>[4x]MGSSHHHHHHSSGGNENLYFQGHMARASGSERHLLLIYTGGTLGMQSKGGVLVPGPGLVTLLRTL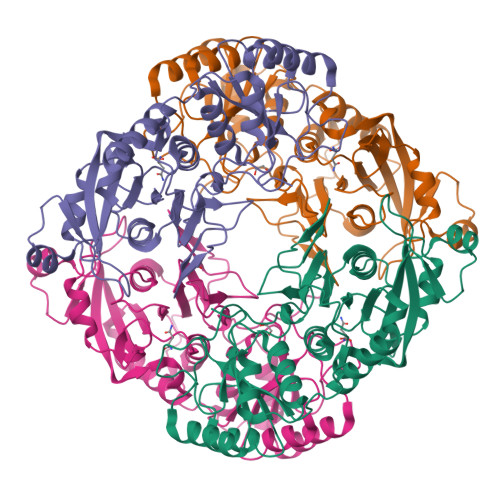PMFHDKEFAQAQGLPDHALALPPASHGPRVLYTVLECQPLLDSSDMTIDDWIRIAKIIERHYEQYQGFVVIHGADTMASGASMLSFMLENLHKPVILTGAQVPIRVLWNDARENLLGALLVAGQYIIPEVCLFMNSQLFRGNRVTKVDSQKFEAFCSPNLSPLATVGADVTIAWDLVRKVKWKDPLVVHSNMEHDVALLRLYPGIPASLVRAFLQPPLKGVVLETFGSGNGPSKPDLLQELRAAAQRGLIMVNCSQCLRGSVTPGYATSLAGANIVSGLDMTSEAALAKLSYVLGLPELSLERRQELLAKDLRGEMTLPTADLHQSSPPGSTLGQGVARLFSLFGCQEEDSVQDAVMPSLALALAHAGELEALQALMELGSDLRLKDSNGQTLLHVAARNGRDGVVTMLLHRGMDVNARDRDGLSPLLLAVQGRHRECIRLLRKAGACLSPQDLKDAGTELCRLASRADMEGLQAWGQAGADLQQPGYDGRSALCVAEAAGNQEVLALLRNLALVGPEVPPAI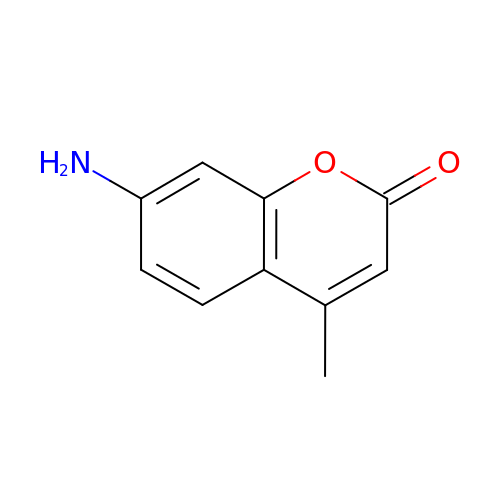7-AMINO-4-METHYL-CHROMEN-2-ONE | C10 H9 N O2 | GLNDAGDHSLMOKX-UHFFFAOYSA-N> SQKNFLCDTGAYELVGAFLENYLREFENDEFRHNLYKYYSENSIFTLTCNYNVVQNHQTPKILQRLSKYNRHARNLRNKDYSKASDGVFFGCTYIVEILLQLPRVTHDFHSLQTDVMHYNGKGAVIYVAGLLRDEPPSTRNGHGSKTDIGGVLLGFSRQFVVTFDEANLGLGKRARRLKIANERLHITNPSKTAIRNAF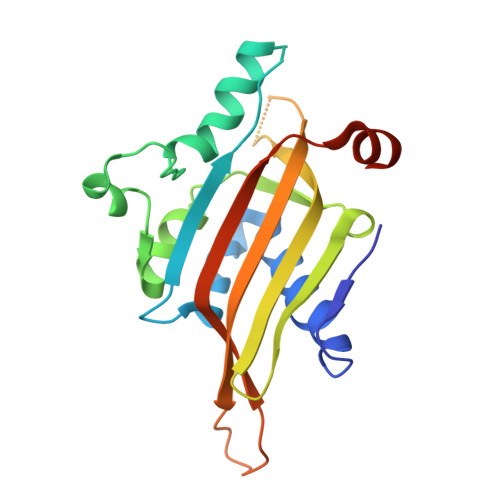SVNFPDP ALPHA-FLUORO-AMIDOCARBOXYMETHYLDETHIA COENZYME A COMPLEX | 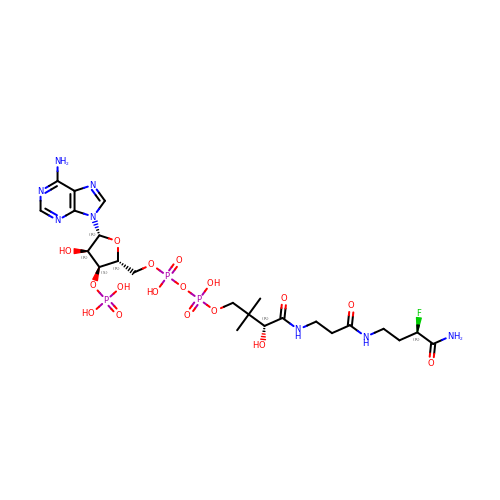C23 H38 F N8 O17 P3 | AXBPCHJFKHSRQL-SYSIYMLXSA-N>GSQSSERVVIGSKPFNEQYILANMIAILLEENGYKAEVKEGLGGTLVNYEALKRNDIQLYVEYTGTAYNVILRKQPPELWDQQYIFDEVKKGLLEADGVVVAAKLGFRDDYALAVRADWAEENGVEKISDLAEFADQLVFGSDPEFASRPDGLPQIKKVYGFEFKEVKQMEPTLMYEAIKNKQVDVIPAYTTDSR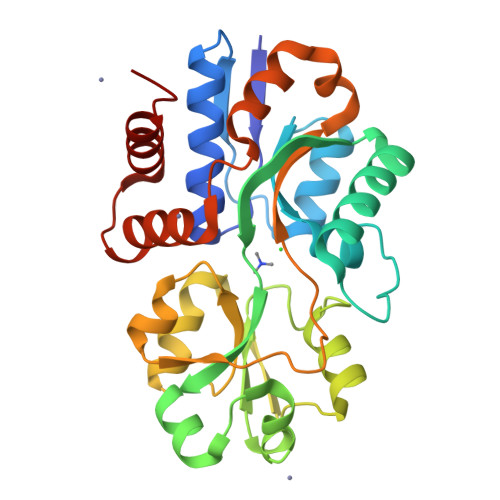VDLFNLKILEDDKGALPPYDAIIIVNGNTAKDEKLISVLKLLEDRIDTDTMRALNYQYDVEKKDAREIAMSFLKEQGLVK[2x]> MHHHHHHSSGRENLYFQGQKDGIFKVMLVGESGVGKSTLAGTFGGLQGDSAHEPENPEDTYERRIMVDKEEVTLVVYDIWEQGDAGGWLRDHCLQTGDAFLIVFSVTDRRSFSKVPETLLRLRAGRPHHDLPVILVGNKSDLARSREVSLEEGRHLAGTLSCKHIETSAALHHNTRELFEGAV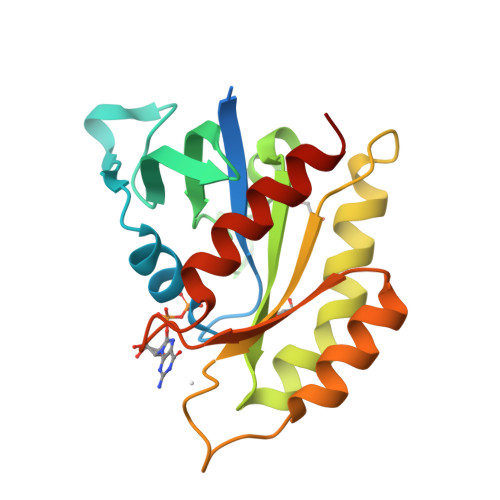RQIRLRRGRNHA> MEQLTKN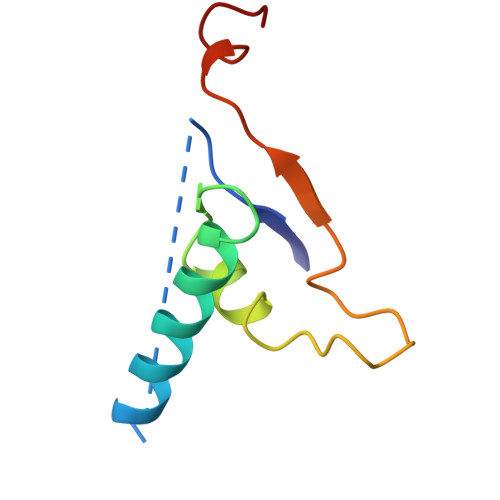QRKKRDEIEAGKSYCSRRFGGATCDDKSAQIYARFDKNDWRIQPAEFYRFHDAEVNTFGYF>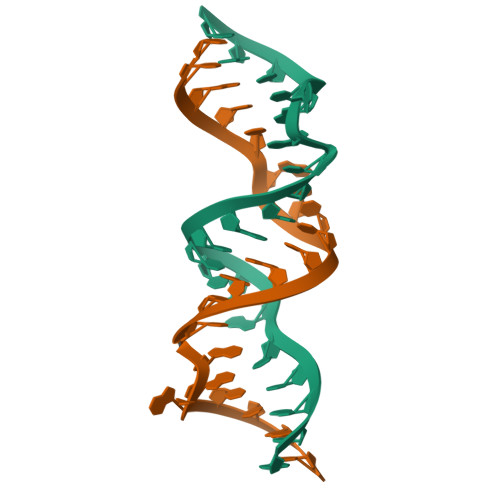GCGUCACCCCGGACAAGUCGC[4x]NDCBE (SLC4A8) mediates Na+-driven Cl‾/CO32‾ exchange and belongs to the Na+-dependent group of the solute carrier family 4 (SLC4) transporters. NDCBE exchanges one Na+ and one CO32‾ ion for one Cl‾ ion4,5. Na+‒driven Cl‾/CO32‾ exchange activity plays an important role in pH regulation in specific cells throughout the brain, kidney and the rest of the body. SLC4 monomers consist of a large C-terminal transmembrane domain (TMD), involved in transport mediation, and a smaller N-terminal cytoplasmic domain (CD).

In this work, we report the cryo-EM 3.4 Å structure of the OF conformation of NDCBE (SLC4A8), which shares transport properties with both AE1 and NBCe1 by mediating the electroneutral exchange of sodium-carbonate with chloride. The cryo-EM map reveals that NDCBE is a dimer with each monomer comprising 14 TMs (TMs 1-14), five amphipathic helices (H1-2, H7-9), and a C-terminal cytoplasmic helix (H10), together with the loops connecting all these helices including the long EL3. The TM helices can be divided into two structural domains, the core domain (TMs 1-4 and TMs 8-11 with H1-2 and H7) and the gate domain (TMs 5-7 and TMs 12-14 with H8-9), which are separated by a cleft on the extracellular side of the protein, providing ion transport cavities between the core domain and the gate domain. TM3, TM10 and the antiparallel β-sheets preceding the two helices in the core domain have been proposed to contribute to substrate coordination in AE110 and NBCe111. This region in our surface-rendered NDCBE atomic model presents as an extracellular-facing cavity where solvent can access from the extracellular side to the ion coordination area, suggesting an outward-facing state (OF). The 3.0 Å resolution cryo-EM map of the core region reveals two densities in this putative ion coordination area, approximately halfway across the membrane, likely corresponding to Na+ and CO32‾. Na+ is coordinated by the hydroxyl oxygens of Thr804 and Thr847 and forms an ionic bond with the carboxyl group of Asp800, with coordination distances of around 2.4 Å, 2.6 Å and 2.6 Å, respectively. A CO32‾ oxygen is coordinated by the backbone amide group of Gly539 and also by the sidechain hydroxyl group of Thr538 with coordination distances of 4.0 Å and 2.9 Å, respectively. In the NDCBE structure, EL3 forms a relatively rigid domain-like structure consisting of four short α-helices (H3‒H6) and one pair of anti-parallel β-strand. EL3 is stabilized by two intramolecular disulfide bonds, Cys636‒Cys684 and Cys638‒Cys672, as well as hydrogen bonds between the anti-parallel β-strand. Dimerization in EL3 is supported by formation of hydrogen bonds between the carbonyl oxygen of Asp629/hydroxyl oxygen of Ser632 and the amidogen nitrogen of Val669 from the neighboring subunits.

>LFGGLVLDVKRKAPWYWSDYRDALSLQCLASFLFLYCACMSPVITFGGLLGEATEGRISAIESLFGASMTGIAYSLFAGQPLTILGSTGPVLVFEKILFKFCKDYALSYLSLRACIGLWTAFLCIVLVATDASSLVCYITRFTEEAFASLICIIFIYEAIEKLIHLAETYPIHMHSQLDHLSLYYCRCALPENPNNHTLQYWKEHSIPTADVNWANLTVSECQEMHGEFIGSACGHHGPYTPDVLFWSCILFFATFIVSSTLKTFKTSRYFPTRVRSTVSDFAVFLTIFTMVILDFLIGVPSPKLQVPSVFKPTRDDRGWFISPIGPNPWWTVIAAIIPALLCTILIFMDQQITAVIINRKEHKLKKGCGYHLDLLVVAIMLGVCSLMGLPWFVAATVLSITHVNSLKLESECSAPGEQPKFLGIREQRVTGLMIFVLMGCSVFMTAVLKFIPMPVLYGVFLYMGVSSLQGIQFFDRLKLFGMPAKHQPDFIYLRHVPLRKVHLFTLVQLTCLVLLWVIKASPAAIVFPMMVLALVFVRKVMDLCFSKRELSWLDDLMPESKKKKLDDAKK[2x]N~2~-[(BENZYLOXY)CARBONYL]-N-[(1S,2S)-2-HYDROXY-1-(4-HYDROXYBENZYL)PROPYL]-L-LEUCINAMIDE 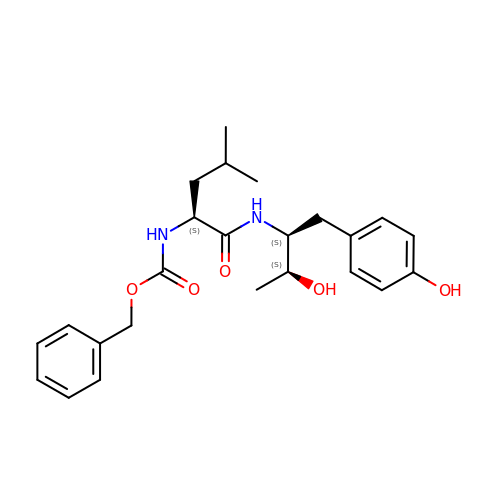| C24 H32 N2 O5 | ZUWYQZGBCBSHFK-HSQYWUDLSA-N(2~{S})-2-(2-fluorophenyl)-2-[4-(2-methylpyrimidin-5-yl)phenyl]-~{N}-oxidanyl-ethanamide 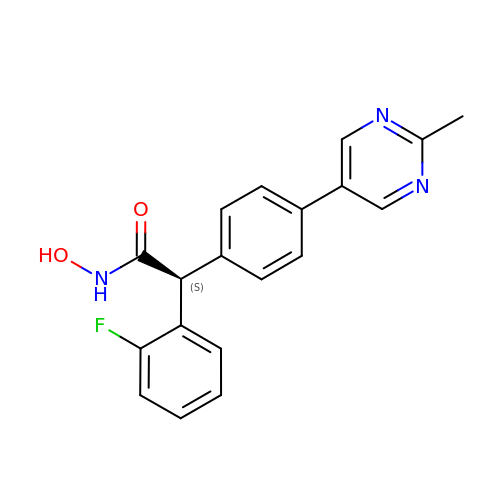| C19 H16 F N3 O2 | SFXMVIQZYOMYOF-SFHVURJKSA-N> AMNTVL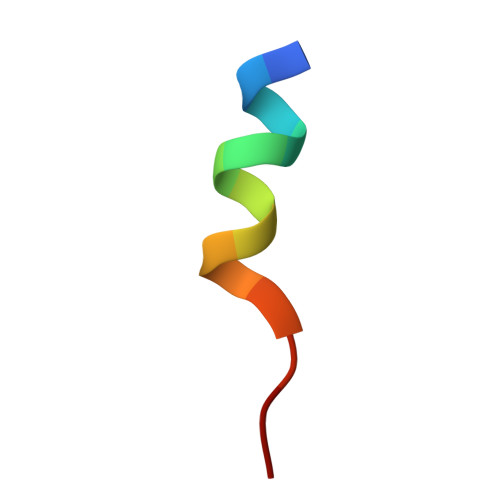ELQKLAHD> GPGSEFRERYELSEKMLSACNLLKYNIKDPKALASKDMRICLNTLQHDWFRVSSQKSAVPAMVGDYIAAFEAVSPDVLRYIINMADGNGNTALHYSVSHSNFQIVKLLLDADVCNVDHQ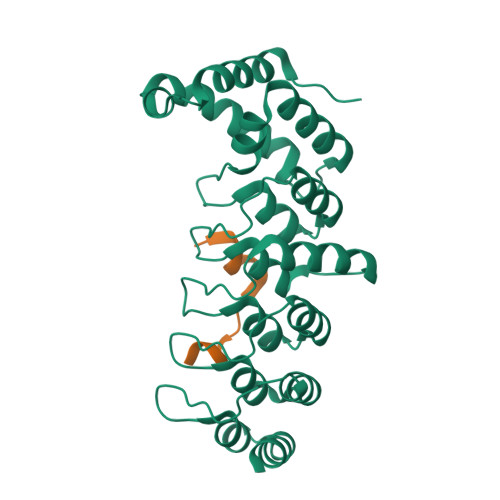NKAGYTPIMLAALAAVEAEKDMQVVEELFSCGDVNAKASQAGQTALMLAVSHGRIDMVKGLLACGADVNIQDDEGSTALMCASEHGHVEIVKLLLAQPGCNGHLEDNDGSTALSIALEAGHKDIAVLLYAHLNFSKAQ;> LMKLCGEVKPKNKARRRTTTQMELLYAD> GPGSLTVGDWLDSIRMGRYRDHFAAGGYSS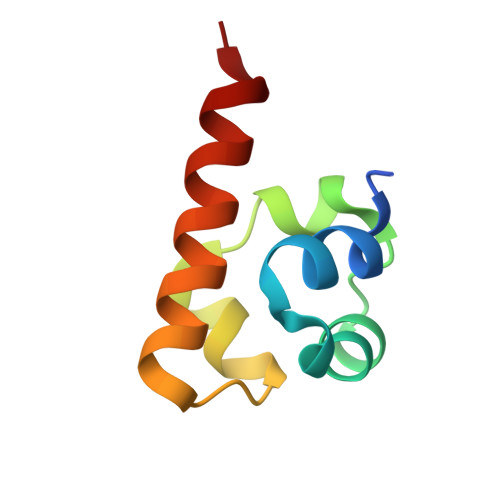LGMVLRMNAQDVRALGITLMGHQKKILGSIQTMRAQLSS>MKLEPLLSDVPRLLMEADLVPVQGTRFQPTGFPDLGAAHYEGPDGRPMLLVESAQSMANRLETVCWDKDADDWVVPLRGLPVVKVLDKAGKPLTNSVLEAHRLNSPYILEGKDKTLFDLLKQELAHMEEGPVDIRKLAETLLKVDANAVLHGVFLAKKELAGGRLRLPRALSAFIEAEDVRVASSGGVKNDHVNPSGDTSRGFGNVPFARDEYVSPRIKAYFNLDLAQIRAFGLGEQVDRLLIALALYKVRRFLVHGLRLRTACDLDCQALRVTRPEGWEVPELSELEAA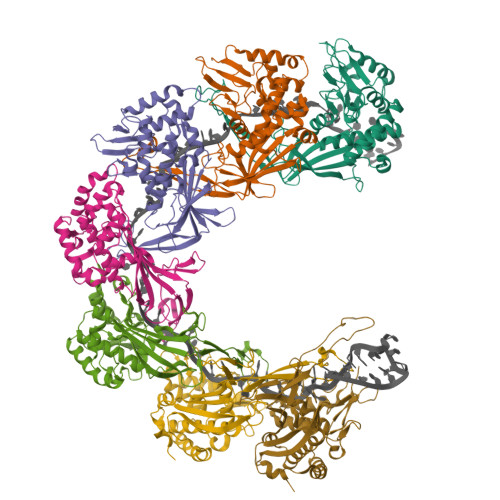LPGLIEAVAGEGRFAQPAVTIVTYEK[7x]The nuclear exosome targeting (NEXT) complex plays a central role in directing non-functional transcripts to exosome-mediated degradation, but the structural and molecular mechanisms remain enigmatic. Here, we elucidated the architecture of the human NEXT complex, showing that it exists as a dimer of MTR4-ZCCHC8-RBM7 heterotrimers. Dimerization preconfigures the major MTR4-binding region of ZCCHC8 and arranges the two MTR4 helicases opposite to each other, with each protomer able to function on many types of RNAs. In terms of architecture, we found that the biological unit of NEXT consists of two copies of each MTR4 and RBM7, assembling symmetrically around a highly intertwined ZCCHC8 homodimer, with an arrangement conducive for targeting different RNA substrates.

Three-dimensional classification followed by 3D refinement and density modification (Terwilliger et al., 2020) led to a reconstruction at a nominal resolution of 4.0 Å, but with a map quality sufficient to trace the ZCCHC8 globular module de novo. This module is formed by the interaction of two ZCCHC8 protomers (referred to as ZCCHC8A and ZCCHC8B), involving their respective dimerization segments (residues 78–198). The dimerization segments of ZCCHC8 intertwine to form a central six-stranded β-sheet characterized by domain swapping: the first β-strands are exchanged between the two ZCCHC8 protomers, resulting in a β3A-β2A-β1B-β1A-β2B-β3B topology of secondary structure elements. Beneath the β-sheet, two α helices from the ZCCHC8 protomers (α2A and α2B), positioned below the corresponding β-strands (β1A and β1B), pack against each other in an antiparallel fashion with conserved hydrophobic interactions (Phe115 and Leu119). Above the β-sheet, the helices at the N terminus of the dimerization segments of the two protomers (α1A and α1B) protrude to form a parallel coiled-coil oriented in a roughly perpendicular fashion with respect to the ZCCHC8 dimerization module. A major interaction is centered at the canonical arch-interacting motif (AIM) of ZCCHC8A (residues 178–184), consistent with biochemical mapping experiments (Lingaraju et al., 2019a). The ZCCHC8 AIM is indeed embedded in strand β3 of the dimerization module and, as such, it appears to be pre-configured in the β-strand conformation with which canonical AIMs are known to recognize the MTR4 KOW domain (Falk et al., 2017b). At the C terminus of the ZCCHC8A AIM, the polypeptide chain makes a 90° bend (residues 185–199). This region is stabilized by a striking array of intramolecular proline-aromatic interactions (Pro142-Pro140-Pro186-Trp198-Pro192), resulting in a “bulge” that contacts a hydrophobic patch on KOWA (MTR4A Pro652, Leu651, and Phe677).

>GPDSENGVGDAELRERLRQCEETIEQLRAENQELKRKLNILTRPSGILVNDTKLDGPILQILFMNNAISKQYHQEIEEFVSNLVKRFEEQQKNDVEKTSFNLLPQPSSIVLEEDHKVEESCAIKNNKEAFSVVGSVLYFTNFCLDKLGQPLLNENPQLSEGWEIPKYHQVFSHIVSLEGQEIQVKAKRPKPHCFNCGSEEHQMKDCPMPRNAARISEKRKEYMDACGEANNQNFQQRYHAEEVEERFGRFKPGVISEELQDALGVTDKSLPPFIYRMRQLGYPPGWLKEAELENSGLALYD[2x];>GPDSMADAFGDELFSVFEGDSTTAAGTKKDKEKDKGKWKGPPGSADKAGKRFDGKLQSESTNNGKNKRDVDFEGTDEPIFGKKPRIEESITEDLSLADLMPRVKVQSVETVEGCTHEVALPAEEDYLPLKPRVGKAAKEYPFILDAFQREAIQCVDNNQSVLVSAHTSAGKTVCAEYAIALALREKQRVIFTSPIKALSNQKYREMYEEFQDVGLMTGDVTINPTASCLVMTTEILRSMLYRGSEVMREVAWVIFDEIHYMRDSERGVVWEETIILLPDNVHYVFLSATIPNARQFAEWICHLHKQPCHVIYTDYRPTPLQHYIFPAGGDGLHLVVDENGDFREDNFNTAMQVLRDAGDLAKGDQKGRKGGTKGPSNVFKIVKMIMERNFQPVIIFSFSKKDCEAYALQMTKLDFNTDEEKKMVEEVFSNAIDCLSDEDKKLPQVEHVLPLLKRGIGIHHGGLLPILKETIEILFSEGLIKALFATETFAMGINMPARTVLFTNARKFDGKDFRWISSGEYIQMSGRAGRRGMDDRGIVILMVDEKMSPTIGKQLLKGSADPLNSAFHLTYNMVLNLLRVEEINPEYMLEKSFYQFQHYRAIPGVVEKVKNSEEQYNKIVIPNEESVVIYYKIRQQLAKLGKEIEEYIHKPKYCLPFLQPGRLVKVKNEGDDFGWGVVVNFSKKSNVKPNSGELDPLYVVEVLLRCSKESLKNSATEAAKPAKPDEKGEMQVVPVLVHLLSAISSVRLYIPKDLRPVDNRQSVLKSIQEVQKRFPDGIPLLDPIDDMGIQDQGLKKVIQKVEAFEHRMYSHPLHNDPNLETVYTLCEKKAQIAIDIKSAKRELKKARTVLQMDELKCRKRVLRRLGFATSSDVIEMKGRVACEISSADELLLTEMMFNGLFNDLSAEQATALLSCFVFQENSSEMPKLTEQLAGPLRQMQECAKRIAKVSAEAKLEIDEETYLSSFKPHLMDVVYTWATGATFAHICKMTDVFEGSIIRCMRRLEELLRQMCQAAKAIGNTELENKFAEGITKIKRDIVFAASLYL[2x]Among these, a notable TFR in Mtb is Mce3R, which is encoded by a gene located upstream of the virulence-associated yrbE3A (mce3) operon and represses genes within the Mce3R regulon. In contrast to a typical TFR gene, the mce3R gene is a fusion of two distinct TFR sequences that encode a double-TFR polypeptide. The genes encoded within the Mce3R regulon play key roles in lipid metabolism, resistance to oxidative stress, and persistence within the host. Additionally, mce3R is encoded in the Mce3R regulon and is thus autoregulated. Here, we report the first three-dimensional structure of a double TFR repressor that folds as an asymmetric Ω and engages with the DNA major groove of an equally asymmetric operator sequence.

The final map for the Mce3R/Probe A complex was reconstructed to a resolution of 2.51 Å. The cryo-EM structure of Mce3R/Probe A revealed that the Mce3R dimer binds to two identical duplexes of DNA. The M1M2 TFR monomer forms a C2-symmetric homodimer, and each protomer binds an oligonucleotide duplex. In agreement with the dissociation constants measured by EMSA, Mce3R is bound to the 27-bp region (region 3) of the Probe A duplex. There is no electron density for regions 1 and 2 in the model. Each 392-amino acid Mce3R monomer is folded into 21 α-helices (α1-α21), and each monomer adopts an omega, Ω, shaped TTR-family fold. A four-helix bundle formed from α-helices α8, α9, α19, and α21 forms the apex of the Ω. One arm of the Ω is formed by M1 and the other arm by M2, resulting in an asymmetric TFR assembly. Thus, the four-helix bundle at the core is assembled from the same protomer, unlike typical TFRs in which each protomer contributes two identical helices. The two nonidentical HTHs from each TFR bind within the high-affinity, nonpalindromic operator motif, with Arg53 and Lys262 inserted into the major groove.

>[2x]MASVAQPVRRRPKDRKKQILDQAVGLFIERGFHSVKLEDIAEAAGVTARALYRHYDNKQALLAEAIRTGQDQYQSARRLTEGETEPTPRPLNADLEDLIAAAVASRALTVLWQREARYLNEDDRTAVRRRINAIVAGMRDSVLLEVPDLSPQHSELRAWAVSSTLTSLGRHSLSLPGEELKKLLYQACMAAARTPPVCELPPLPAGDAARDEADVLFSRYETLLAAGARLFRAQGYPAVNTSEIGKGAGIAGPGLYRSFSSKQAILDALIRRLDEWRCLECIRALRANQQAAQRLRGLVQGHVRISLDAPDLVAVSVTELSHASVEVRDGYLRNQGDREAVWIDLIGKLVPATSVAQGRLLVAAAISFIEDVARTWHLTRYAGVADEISGLALAILTSGAGNLLRA>MTEVNAFADTPWRAGVIQDFARSELFDRTFEEGMQLVEETAAYLDGAGRHDSKVLSRNAALGYATESMRLTTRLMQVASWLLVQRAVREGEMPPEAACAEAYRLAEEAPADGPAVEELPFGLMNLLQRSERLYERVRHLDRR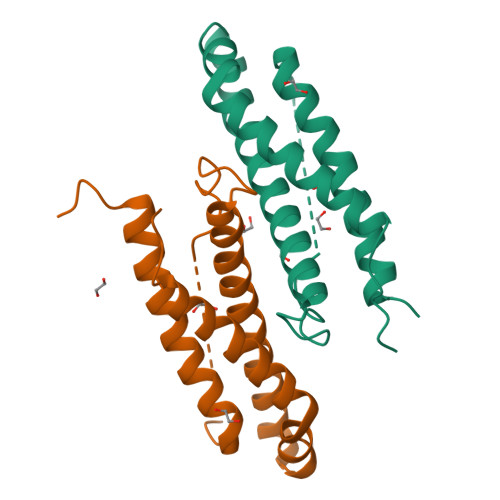MYVESPNEEAPRPVQNQLDRLTAAFGG[2x]[1,2,4]triazolo[3,4-b][1,3]benzothiazol-6-ol | C8 H5 N3 O S | 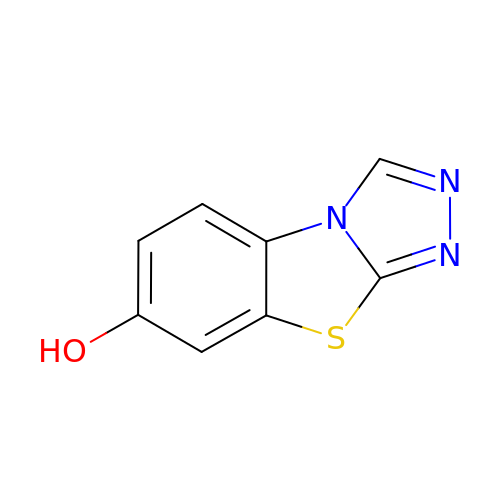IWIXTZQBCXYDRG-UHFFFAOYSA-N>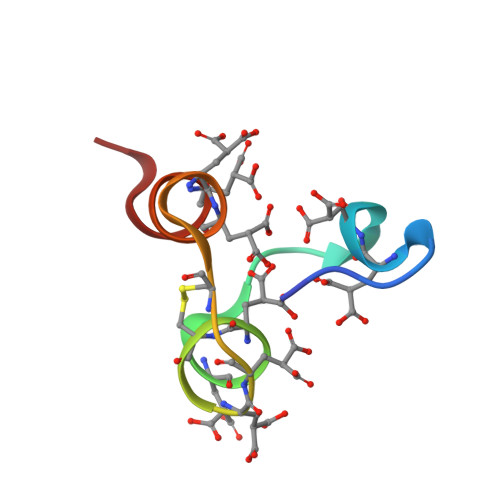 ANSFLEELRHSSLERECIEEICDFEEAKEIFQN[(2~{S})-2-methylpiperidin-1-yl]-morpholin-4-yl-methanone 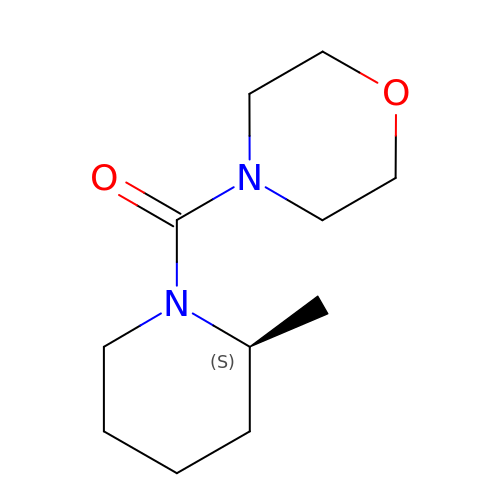| C11 H20 N2 O2 | FLEIZTSEYWQEHP-JTQLQIEISA-N>[2x]MKDSTYSKLNPRLLKIWRNYLNMNKYKVSYKGPGPGVKFSVEALRCHLRDHVNVSMIEATDFPFNTTEWEGYLPKENFRTKVGPWQRCAVVSSAGSLKNSQLGREIDNHDAVLRFNGAPTDNFQQDVGSKTTIRLMNSQLVTTEKRFLKDSLYTEGILIVWDPSVYHADIPKWYQKPDYNFFETYKSYRRLNPSQ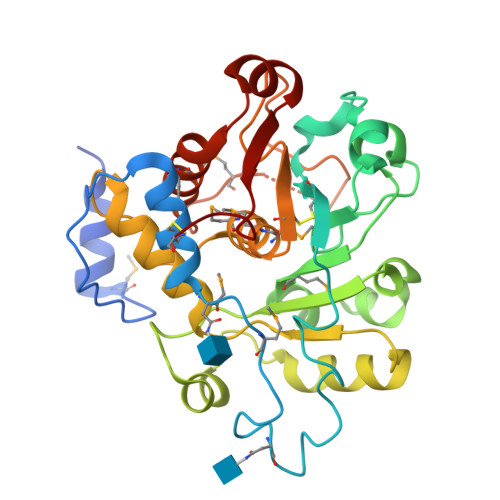PFYILKPQMPWELWDIIQEISADLIQPNPPSSGMLGIIIMMTLCDQVDIYEFLPSKRKTDVCYYHQKFFDSACTMGAYHPLLFEKNMVKHLNEGTDEDIYLFGKATLSGFRNIRC>MASMYNSDGWYMGEAINMASLNTCAADLGKWQNFIDDYTSNDYYKGTPYIDWVFASSPKGDRWQMNEWSVSEMLKVGGTYEEGGLNCMGFVWHAIAKGLSVESGLDISQTGQYVPFSSYFNGLGLSRKCWATPGGSGGWTVFVDYYNLHYYEFPTKEEMLSSGVLQKGDIIWCVDGSVGLGMAGLRTIADNHHIGIYTGNGTSDSWWQSGPVKADGDLVNVGTDVCPIYGAAAKNTYVVLPWAKKA[2x]

R. flavefaciens FD-1 is a gram-positive cellulosome-producing anaerobic bacterium that possesses the most elaborate cellulosome system thus far discovered in nature. The parent protein, RflaF_05439 (accession number: ZP_06142651), consists of a tandem repeat of two conserved modules at the N terminus and a C-terminal XDoc, which also binds to ScaE-Coh (unpublished results). In silico analysis of the structure implied that the protein belongs to an established superfamily of cysteine-like peptidases, termed NlpC/P60, and this domain will hereafter be coined NlpC/P60_2. The NlpC/P60 superfamily of peptidases is characterized by a conserved catalytic triad, which contains cysteine, histidine and a polar residue (i.e., glutamine, aspargine, histidine, glutamate or aspartate) within a catalytic core.

The X-ray crystal structure of the second module of the tandem repeat of RflaF_05439 from R. flavefaciens FD-1 was determined at a resolution of 1.38 Å. There are no significant differences between the two molecules in the asymmetric unit (RMSD of 0.06 Å for all Cα atoms). The overall fold consists of two globular domains that form a tight interface: an N-terminal α-helical domain and a C-terminal domain comprised of 6 antiparallel βstrands covered by short α-helices and loops. The potential active site of NlpC/P60_2 is located in the channel groove that runs along the interface between the N-and C-terminal domains. The crystal structure of the protein module described in this work allows the assignment of a putative function for the RflaF_05439 protein, which is identified to be a member of the NlpC/P60 superfamily, possessing the characteristic conserved catalytic triad residues (Cys109/His215/Gln230). A fourth residue, Tyr71, is also conserved. This residue is important for formation of a putative oxyanion hole, which helps stabilize transitional forms between the peptidase and the substrate. In the NlpC/P60_2 structure, extra electron density was discovered contiguous with the side chain of the catalytic cysteine, Cys109. This extraneous electron density was modeled as acetate. In any case, is it likely that the modified cysteine would lead to an inactivated enzyme, which may explain why attempts to demonstrate protease activity were unsuccessful.>KFRTMRQNLQEASDVLDDQIESFTKIIQNHYKLSPNDFADPTIQSQSEIYAVGRIVPDSPTYDKFLNPESLSLETSRMGGVGRRVRLDLSQVNELSFFLGQIVAFKGKNANGDYFTVNSILPLPYPNSPVSTSQELQEFQANLEGSSLKVIVTCGPYFANDNFSLELLQEFIDSINNEVKPHVLIMFGPFIDITHPLIASGKLPNFPQFKTQPKTLDELFLKLFTPILKTISPHIQTVLIPSTKDAISNHAAYPQASLIRKALQLPKRNFKCMANPSSFQINEIYFGCSNVDTFKDLKEVIKGGTTSSRYRLDRVSEHILQQRRYYPIFPGSIRTRIKPKDVSTKKETNDMESKEEKVYEHISGADLDVSYLGLTEFVGGFSPDIMIIPSELQHFARVVQNVVVINPGRFIRATGNRGSYAQITVQCPDLEDGKLTLVEGEEPVYLHNVWKRARVDLIAS[4x];>NLQPLETTITDVERFKDTVTLELSCPSCDKRFPFGGIVSSNYYRVSYNGLQCKHCEQLFTPLQLTSQIEHSIRAHISLYYA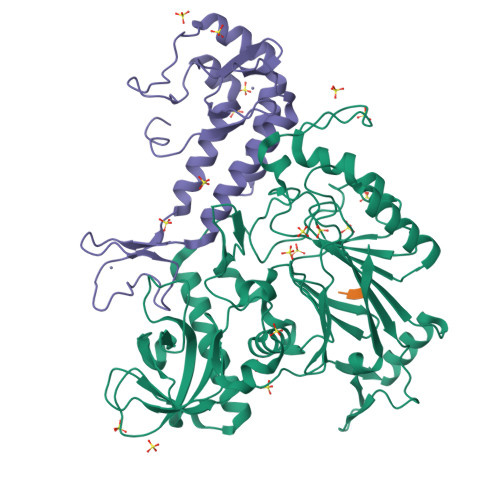GWLQCDDSTCGIVTRQVSVFGKRCLNDGCTGVMRYKYSDKQLYNQLLYFDSLFDCEKNKKQELKPIYLPDDLDYPKEQLTESSIKALTEQNRELMETGRSVVQKYLNDCGRRYVDMTSIFDFMLN[4x]>GPLGSQQLTIEVLVTVDGVNFRTVVLNNKNTYRSQLGCVFFNGADISDTIPDEKQNGHSLYLADNLTADETKALKELYGPVDPTFLHRFYSLKAAVHKWKMVVCDKVRSLKLSDNNCYLNAVIMTLDLLKDIKFVIPALQHAFMKHKGGDSTDFIALIMAYGNCTFGAPDDASRLLHTVLAKAELCCSARMVWREWCNVCGIKDVVLQGLKACCYVGVQTVEDLRA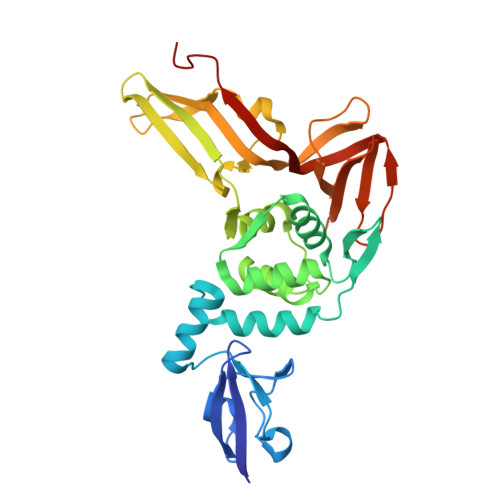RMTYVCQCGGERHRQIVEHTTPWLLLSGTPNEKLVTTSTAPDFVAFNVFQGIETAVGHYVHARLKGGLILKFDSGTVSKTSDWKCKVTDVLFPGQKYSSDCNVVRYSLDG[2x]>MARRNRRLSSASVYRYYLKRISMNIGTTGHVNGLSIAGNPEIMRAIARLSEQETYNWVTDYAPSHLAKEVVK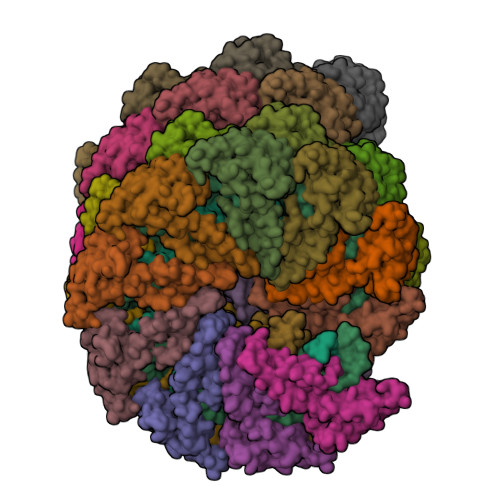QISGKYNIPGAYQGLLMAFAEKVLANYILDYKGEPLVEIHHNFLWELMQRQSGAGLGVTSGFIYTFVRKDGKPVTVDMSKVLTEIEDALFKLVKK[17x];>MAGRQSHKKIDVRNDTSTRYKGKLYGIFVNYMGEKYAQQLVENMYSNYNDVFVEIYNKMHNALRPTLVKLAGAGATFPLWQLVNEAIYAVYLTHKETASFLVTKYVARGVPAMTVKTLLAEVGNQLKELVPAVAEQIGSVTLDHTNVVSTVDNIVTSMPALPNSYAGVLMKTKVPTVTPHYAGTGTFSSMESAYKALEDIERGL[17x]> D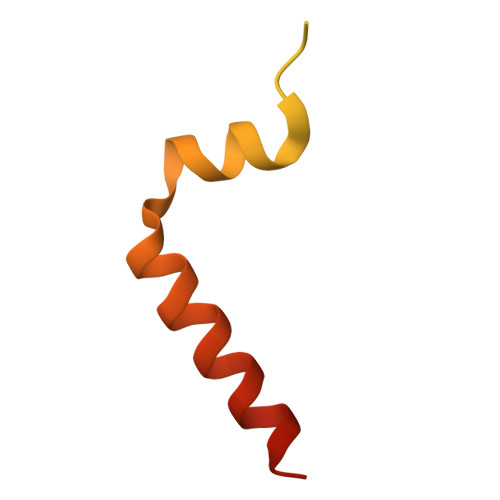LAPRQIARYRTDNGEEFEVPFADDAEIPGTWLCRNGMEGTLIEGDLPEPKKVKPPRTHWDMLLERRSIEELEELLKERLELIRSRRRG> MENGEAKQSVPLLTPYKMGRFNLSHRVVLAPLTRQRSYGNVPQPHAAIYYSQRTTPGGFLITEATGVSD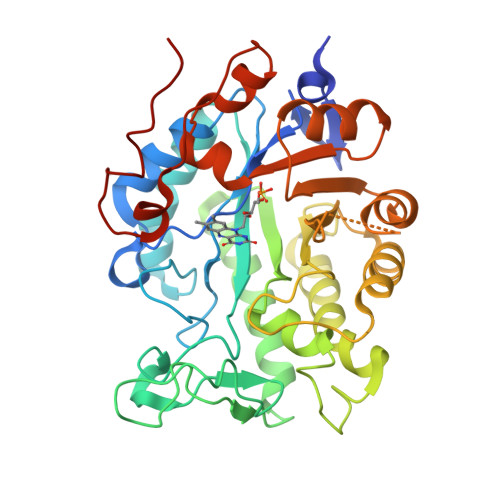TAQGYQDTPGIWTKEHVEAWKPIVDAVHAKGGIFFCQIWHVGRVSNSGFQPNGKAPISCSDKPLMPQIRSNGIDEALFTPPRRLGIEEIPGIVNDFRLAARNAMEAGFDGVEIHGANGYLIDQFMKDTVNDRTDEYGGSLQNRCKFPLEIVDAVAKEIGPDRVGIRLSPFADYMESGDTNPGALGLYMAESLNKYGILYCHVIEARMKTMGEVHACPHTLMPMRKAFKGTFISAGGFTREDGNEAVSKGRTDLVAYGRWFLANPDLPKRFQVDAPLNKYDRPTFYTSDPVVGYTDYPFLESTA> GPDSMGAAAAEADRTL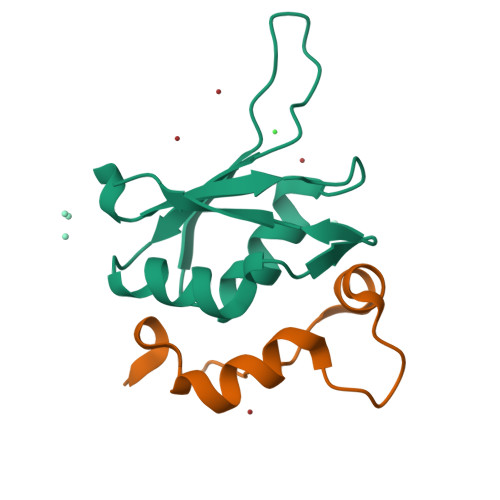FVGNLETKVTEELLFELFHQAGPVIKVKIPKDKDGKPKQFAFVNFKHEVSVPYAMNLLNGIKLYGRPIKIQFRS;> GPDSMRFKPGVISEELQDALGVTDKSLPPFIYRMRQLGYPPGWLK2-bromobenzoic acid | C7 H5 Br O2 | 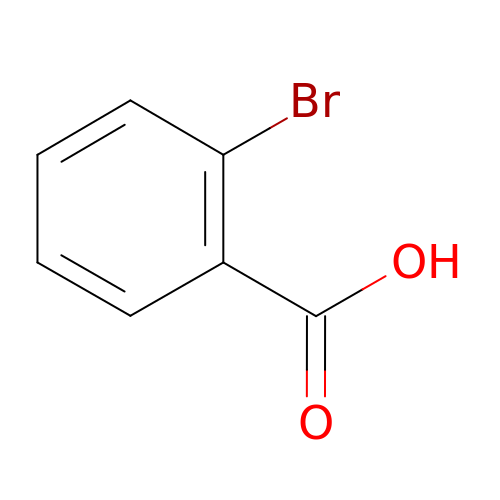XRXMNWGCKISMOH-UHFFFAOYSA-N>[4x]MRLNDPVHYDGAWHVYKYSDVKHVLMNDKIFSSNPGNRYSNAGGISFITMDNPEHKEFRDISAPYFLPSKINDYKDFIEETSNDLIKNIDNKDIISEYAVRLPVNIISKILGIPD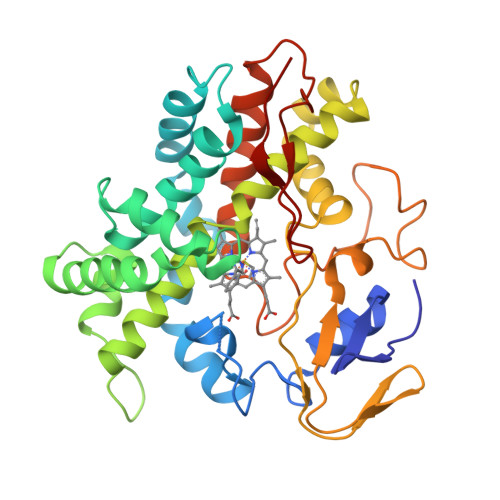SDMPLFKLWSDYIIGNKRDENFNYVNNRMVSRLLEIFKSDSHGIINVLAGSSLKNRKLTMDEKIKYIMLLIIGGNETTTNLIGNMIRVIDENPDIIDDALKNRSGFVEETLRYYSPIQFLPHRFAAEDSYINNKKIKKGDQVIVYLGSANRDETFFDEPDLFKIGRREMHLAFGIGIHMCLGAPLARLEASIALNDILNHFKRIKIDYKKSRLLDNKMVLGYDKLFLS>GAMGEASHDSAESLVAARAEKVANLYRWLDTDNDVATDKYVPVPGFERVDVDVSDEVKQRMIQSMSGYIEHTDNQVPKDQAEALATLFVESTLDYDWDKRVEFLTKLESYGYSFEAPHAEKSIVSFWSGKNFKQYRDILDNAQTDGKKVVYDIDVKGNAFAIDLNKHLMRWGGLFLDPDNAEQNQLKSSIDAATFSNTGFWSSVYATGAQNDVYVIAEGGVRLGNYFWNVELPALRQLQREGLVGEIRLLDKPVSEYKDLPADQIGRRLTDAGVAVKVRFDALSHERQAELLADNPDGYKADTLVELDVKLSAIDSMLRES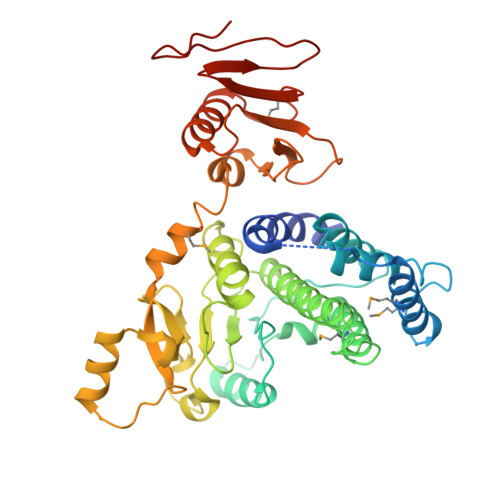LPFYSLRTERNLLVQEGEEGFEVRSWPGIDGKSKTILLDNPEDAAQQKSIERFILANFDNFEQMPDELFLVDNKVLSHHDGRTRIIAQKEDGAWTYNT[2x]>[2x]MSAELASRGRKVYFVGLNEYPFLPLVAGLLRTYAEQDERIAAAYDFQEPVFLVAPVQEMA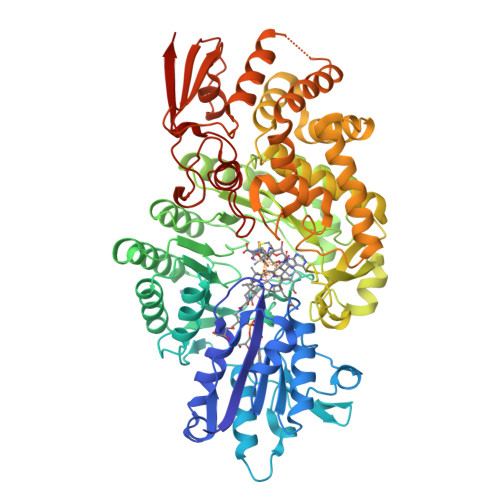DGIVEPDVLALSCYVWNFRRQMKVAKLVKERYPNVLVVAGGPHVPDRPGNFFEKHPYVDVLAHGEGEVAFRELLATRLSDHPDYTAVPGVSVRRGTEAVVGPKAKRLPRLIDTPSPYLLGVMDGAVATCRERGLRFYALWETNRGCPYSCSFCDWGSATMSTLRKFEDERLQDEIEWFARHDVEDLFICDANFGIMPRDLEIAHALAEARGELGAPRQVRVNFAKNSNDRVFDISKTWHDADLLMGTTLSMQSTDMDVLEAIDRKNIGLDNYRKLQQRYAAENIHTYTELILGLPMETARSFRDGIGSLLEAGNHEDLRVYELGILPNAPLNTPEKIEQYGLRTVPKRMYVERPGTPDDEAETFEMVMETNAMPRDAWVESFSFIQAVQFLHNGCYTRYLSIFLRQEHGIGYTRFYEGLQDYFTGRPDTVLGALYLRMRSLYHDYIDMPALPLANLVASQPDMAADLAPYGRRRGWTIDNWGWLRIATDFDRFHTELREYLATLGLDPAGDARLEDVLRFQQDVMLRPDYSPELGKSAEYAHDWPGYFAGGLLRPRRVRVAYGDQSFGANGRYRPVPGDLKAFTMAAIGTSYPVSRMGHFCHRFESAEVTSLAEPVVSEQW> MKKVKLIGTLDYGKYRYPKNHPLKIPRVSLLLRFKDAMNLIDEKELIKSRPATKEELLLFHTEDYINTLMEAERSQSVPKGAREKYNIGGYENPVSYAMFTGSSLATGSTVQAIEEFLKGNVAFNPAGGMHHAFKSRANGFCYINNPAVGIEYLRKKGFKRILYIDLDAHHCDGVQEAFYDTDQVFVLSLHQSPEYAFPFEKGFLEEIGEGKGKGYNLNIPLPKGLNDNEFLFALEKSLEIVKEVFEPEVYLLQLGTDPLLEDYLSKFNLSNVAFLKAFNIVREVFGEGVYLGGGGYHPYALARAWTLIWCELSGREVPEKLNNKAKELLKSIDFEEFDDEVDRSYMLETLKDPWRGGEVRKEVKDTLEKAK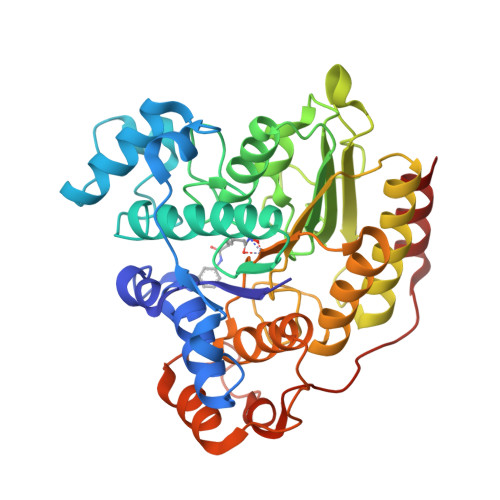ASS N-((1S,2R)-3-(((1S)-2-(CYCLOHEXYLAMINO)-1--METHYL-2-OXOETHYL)AMINO)-2-HYDROXY-1-(PHENYLMETHYL)PROPYL)-3-(ETHYLAMINO)-5-((METHYLSULFONYL)(PHENYL)AMINO)BENZAMIDE 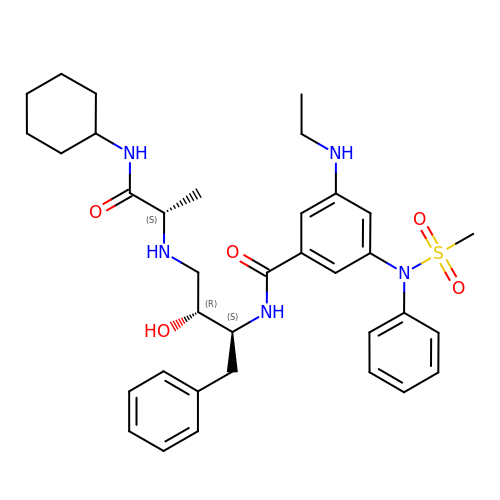| C35 H47 N5 O5 S | SMMANAWVXZZNER-DZMJNENTSA-N>[2x]VTTAGPPVKGRATRQRAAVSAALQEVEEFRSAQELHDMLKHKGDAVGLTTVYRTLQSLADA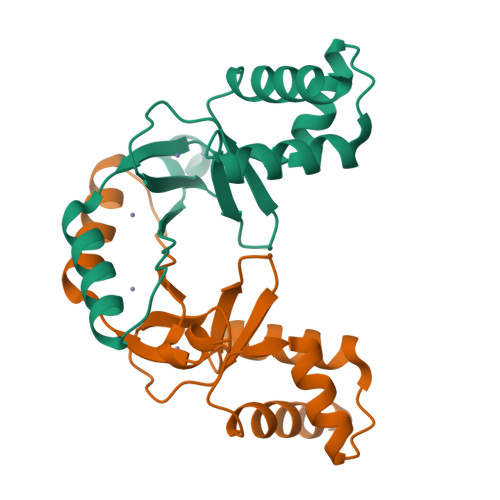GEVDVLRTAEGESVYRRCSTGDHHHHLVCRACGKAVEVEGPAVEKWAEAIAAEHGYVNVAHTVEIFGTCADCAGASGG> MNGIDDLLNINDRIKQVQNERNELASKLQNLKQSLASNDTEVALSEVIAQDIIEVGASVEGLEQLRAKYGDLQILNKLEKVAVQQTQMQAGVDKLDSFERQLDELAEQPPDQFTLDDVKALHSKLTSVFATVPQINNIDSQYAAYNKLKSKVTGKYNDVIIQRLATNWSNTFDQKLLEAQWDTQKFASTSVGLVKCLRENSTKLYQLSLLYLPLEEETQNGDSERPLSRSNNNQEPVLWNFKSLANNFNVRFTYHFHATSSSSKIETYFQFLNDYLAENLYKCINIFHDDCNGLTKPVIHEQFINYVLQPIRDKVRSTLFQNDL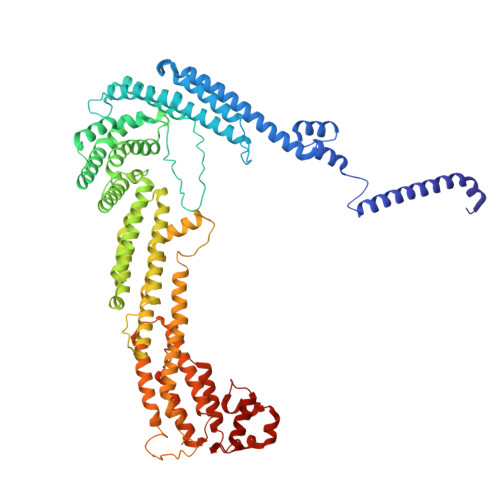KTLIVLISQILATDKNLLNSFHYHGLGLVSLISDEVWEKWINYEVEMANRQFINITKNPEDFPKSSQNFVKLINKIYDYLEPFYDLDFDLLVRYKLMTCSLIFMNLTSSYLDYILTVDSLNETRTKEQELYQTMAKLQHVNFVYRKIKSLSSNFIFIQLTDIVNSTESKKYNSLFQNVENDYEKAMSTDMQNSIVHRIQKLLKETLRNYFKISTWSTLEMSVDENIGPSSVPSAELVNSINVLRRLINKLDSMDIPLAISLKVKNELLNVIVNYFTESILKLNKFNQNGLNQFLHDFKSLSSILSLPSHATNYKCMSLHELVKILKLKYDPNNQQFLNPEYIKTGNFTSLKEAYSIKYLKDTKIQDALYRIIYGNIL>[4x]SMASSGMTRRDPLANKVALVTASTDGIGFAIARRLAQDGAHVVVSSRKQQNVDQAVATLQGEGLSVTGTVCHVGKAEDRERLVATAVKLHGGIDILVSNAAVNPFFGSIMDVTEEVWDKTLDINVKAPALMTKAVVPEMEKRGGGSVVIVSSIAAFSPSPGFSPYNVSKTALLGLTKTLAIELAPRNIR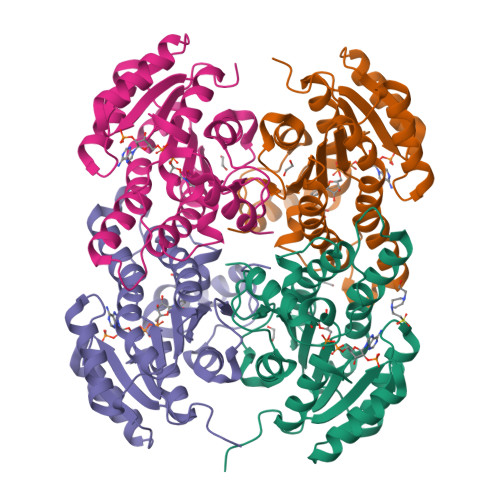VNCLAPGLIKTSFSRMLWMDKEKEESMKETLRIRRLGEPEDCAGIVSFLCSEDASYITGETVVVGGGTPSRL>[4x]MKVAENQK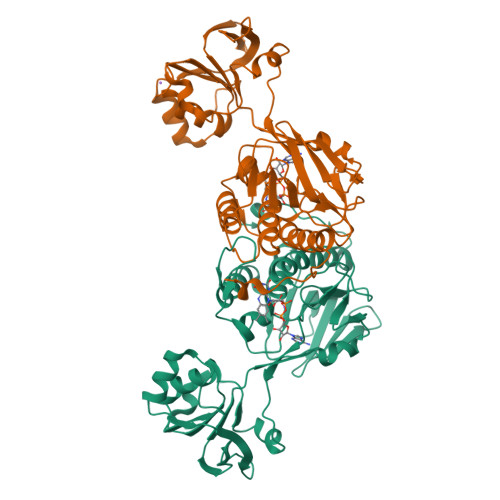VYDITIIGGGPTGLFTAFYGGMRQASVKIIESLPQLGGQLSALYPEKYIYDVAGFPKVRAQELVDNLKEQMKKFDPTVCLEEAVDTLEKQADGIFKLVTNKQTHYSKSVIITAGNGAFQPRRLELEGTAKYEKKNLHYFVDDMNKFAGKRVVVFGGGDSAVDWTMMLEPIAEKVTIVHRRDKFRAHEHSVENLMNSRAEVSTPYVPVELIGDDKIEQVVLQHVKTEEKVIIDVDDVIVNYGFVSSLGPIKNWGLDIQKNSILVNSKMETNIPGIYAAGDICTYEGKVKLIACGFGEAPTAVNNAKAYFDPNAKLQPMHSSSMF> MKILVAVKQTAALEEDFEIREDGMDVDEDFMMYDLNEWDDFSLEEAMKIKESSDTDVEVVVVSVGPDRVDESLRKCLAKGADRAVRVWDDAAEGSDAIVVGRILTEVIKKEAPDMVFAGVQSSDQAYASTGISVASYLNWPHAAVVADLQYKPGDNKAVIRRELEGGMLQEVEINCPAVLTIQLGINKPRYASLRG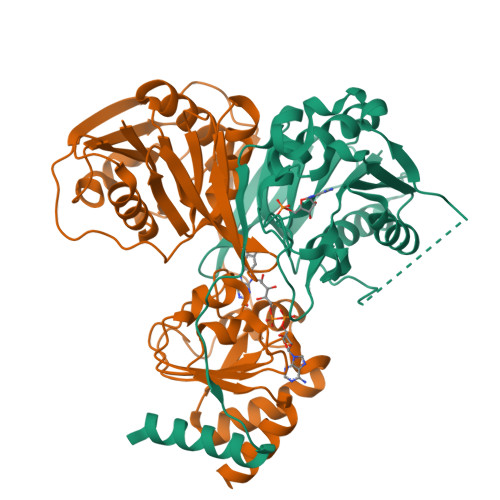IKQAATKPIEEVSLADIGLSANDVGAAQSMSRVRRMYIPEKGRATMIEGTISEQAAKIIQIINEFKGA;> MSKILVIAEHRRNDLRPVSLELIGAANGLKKSGEDKVVVAVIGSQADAFVPALSVNGVDELVVVKGSSIDFDPDVFEASVSALIAAHNPSVVLLPHSVDSLGYASSLASKTGYGFATDVYIVEYQGDELVATRGGYNQKVNVEVDFPGKSTVVLTIRPSVFKPLEGAGSPVVSNVDAPSVQSRSQNKDYVEVGGGNDIDITTVDFIMSIGRGIGEETNVEQFRELADEAGATLCCSEPIADAGWLPKSRQVGQSGKVVGSCKLYVAMGISGSIQHMAGMKHVPTIIAVNTDPGASIFTIAKYGIVADIFDIEEELKAQLAA>MGTKLKKSNNDITIFSENEYNEIVEMLRDYSNGDNLEFEVSFKNINYPNFMRITEHYINITPENKIESNNYLDISLIFPDKNVYRVSLFNQEQIGEFITKFSKASSNDISRYIVSLDPSDDIEIVYKNRGSGKLIGIDNWAITIKSTEEIPLVAGKSKISKPKITGSER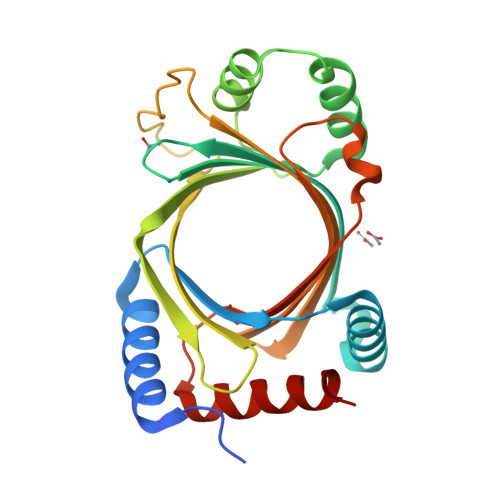IMYRYKTRYSFTINKNSRIDITDVKSSPIIWKLMTVPSNYELELELINKIDINTLESELLNVFMIIQD[2x]>RKPKTGILMLNMGGPETLGDVHDFLLRLFLDRDLMTLPIQNKLAPAIAKRRTPKIQEQYRRIGGGSPIKIWTSKQGEGMVKLLDELSPNTAPHKYYIGFRYVHPLTEEAIEEMERDGLERAIAFTQYPQYSCSTTGSSLNAIYRYYNQVGRKPTMKWSTIDRWPTHHLLIQCFADHILKELDHFPLEKRSEVVILFSAHSLPMSVVNRGDPYPQEVSATVQKVMERLEYCNPYRLVWQSKVGPMPWLGPQTDESIKGLCERGRKNILLVPIAFTSD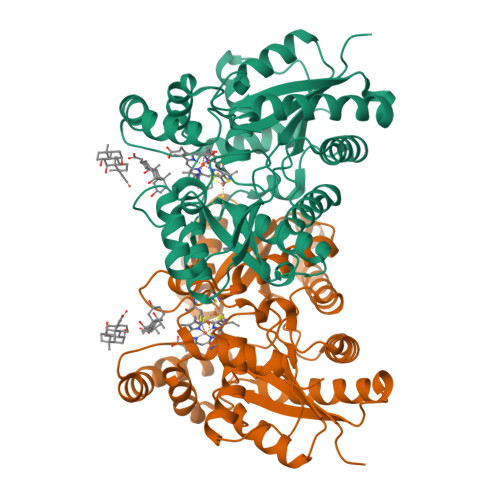HIETLYELDIEYSQVLAKECGVENIRRAESLNGNPLFSKALADLVHSHIQSNELCSKQLTLSCPLCVNPVCRETKSFFTSQQL[2x]>MDFYYLPGSAPCRSVLMTAKALGIELNKKLLNLQAGEHLKPEFLKINPQHTIPTLVDGDFALWESRAIMVYLVEKYGKTDSLFPKCPKKRAVINQRLYFDMGTLYKSFADYYYPQIFAKAPADPELFKKIETAFDFLNTF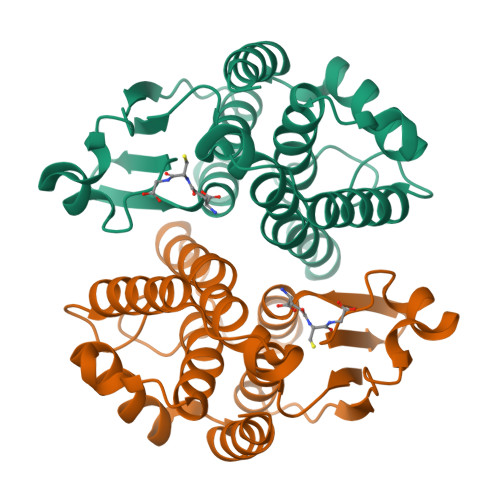LKGHEYAAGDSLTVADLALLASVSTFEVASFDISKYPNVAKWYANLKTVAPGWEENWAGCLEFKKYFG[2x]bis[2-methyl-5-(trifluoromethyl)pyrazol-3-yl]-bis(oxidanyl)boranuide 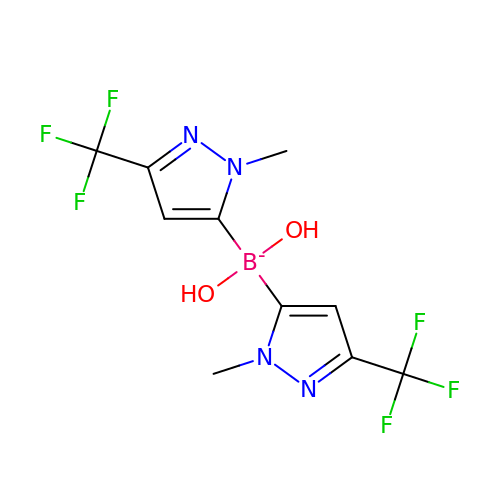| C10 H10 B F6 N4 O2 | XCHJAGXOPCFIKR-UHFFFAOYSA-N>[2x]QAQITGRPEWIWLALGTALMGLGTLYFLVKGMGVS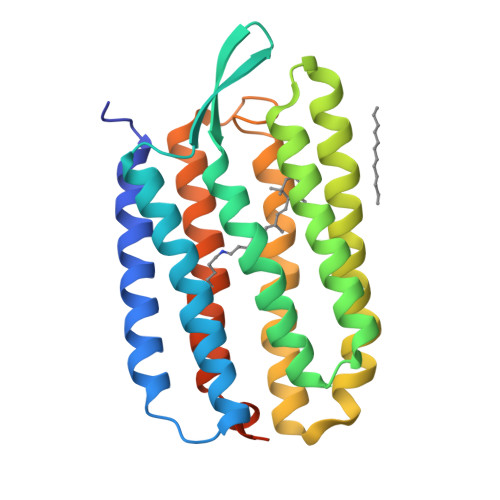DPDAKKFYAIATLVAAIAFTMYLSMLLGYGLTMVPFGGEQNPIYWARYADWLFTTPLLLLDLALLVDADQGTILALVGADGIMIGTGLVGALTKVYSYRFVWWAISTAAMLYILYVLFFGFTSKAESMRPEVASTFKVLRNVTVVLWSAYPVVWLIGSEGAGIVPLNIETLLFMVLDVSAKVGFGLILLRSRAIFGEAEAPEPSAGDGAAATSD>[4x]HHHHHHSSGLVPRGSHMELHAITDDSKPVEELARIIITIQNEVDFIHIRERSKSAADILKLLDLIFEGGIDKRKLVMNGRV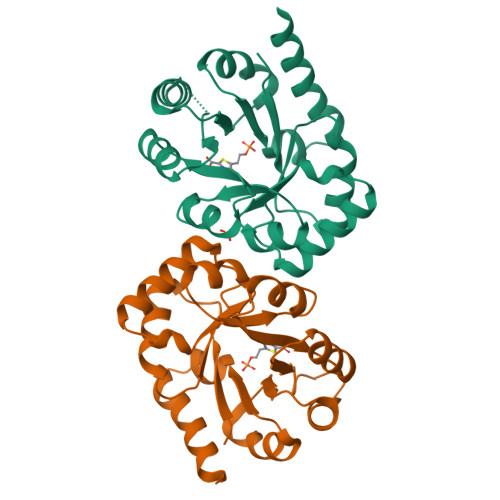DIALFSTIHRVQLPSGSFSPKQIRARFPHLHIGRSVHSLEEAVQAEKEDADYVLFGHVFETDCKKGLEGRGVSLLSDIKQRISIPVIAIGGMTPDRLRDVKQAGADGIAVMSGIFSSAEPLEAARRYSRKLKEMRYEKAL> NVLTVYSPYQSNLIRPILNEFEKQEHVKIEIKHGSTQVLLSNLHNEDFSERGDVFMGGVLSETIDHPEDFVPYQDTSVTQQLEDYRSNNKY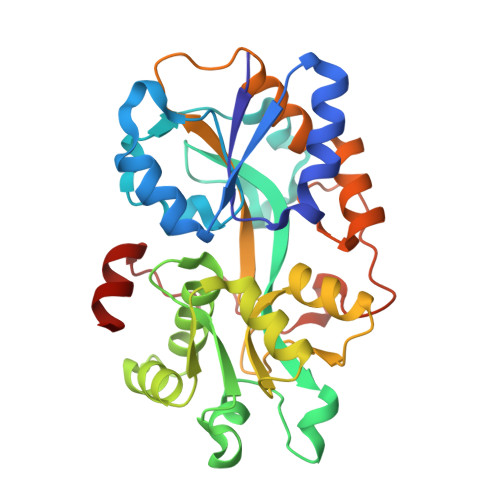VTSFLLMPTVIVVNSDLQGDIKIRGYQDLLQPILKGKIAYSNPNTTTTGYQHMRAIYSMHHRVSDVHQFQNHAMQLSKTSKVIEDVAKGKYYAGLSYEQDARTWKNKGYPVSIVYPIEGTMLNVDGIALVKNAHPHPKRKKLVQYLTSRSVQQRLVAEFDAKSIRKDVSEQSDQSIENLKNIPLIPKSKLPDIPHHKFLEMIQ>MFKKFDEKENVSNCIQLKTSVIKGIKNQLIEQFPGIEPWLNQIMPKKDPVKIVRCHEHIEILTVNGELLFFRQREGPFYPTLRLLHKYPFILPHQQVDKGAIKFVLSGANIMCPGLTSPGAKLYPAAVDTIVAIMAAGAAHALCVGVMKMSAEDIEKVNKGIGIENIHYLNDGLWHMK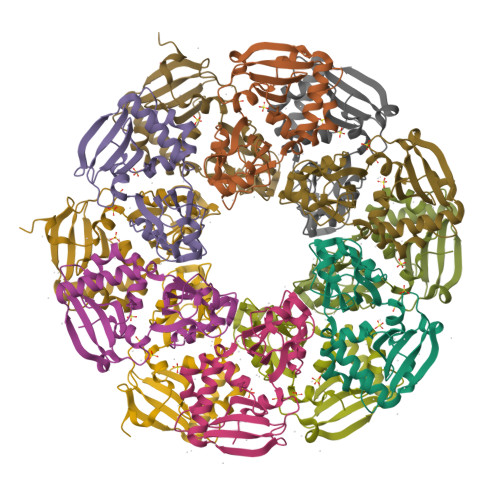TYKAHHHHHH[12x]>AGVAKFAKYPLTFGPSPISNLNRLSQHLGSKVNVYAKREDCNSGLAFGGNKLRK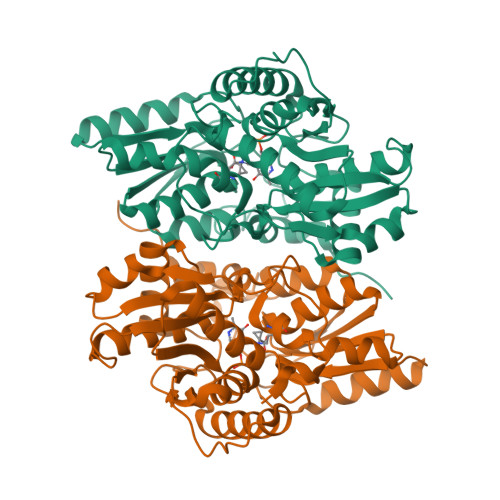LEYIVPDIVEGDYTHLVSIGGRQSNQTRMVAALAAKLGKKCVLIQEDWVPIPEAEKDVYNRVGNIELSRIMGADVRVIEDGFDIGMRKSFANALQELEDAGHKPYPIPAGCSEHKYGGLGFVGFADEVINQEVELGIKFDKIVVCCVTGSTTAGILAGMAQYGRQDDVIAIDASFTSEKTKEQTLRIANNTAKLIGVEHEFKDFTLDTRFAYPCYGVPNEGTIEAIRTCAEQEGVLTDPVFEGKSMQGLIALIKEDYFKPGANVLYVHLGGAPALSAYSSFFPTKTA[4x]> HHHHHHS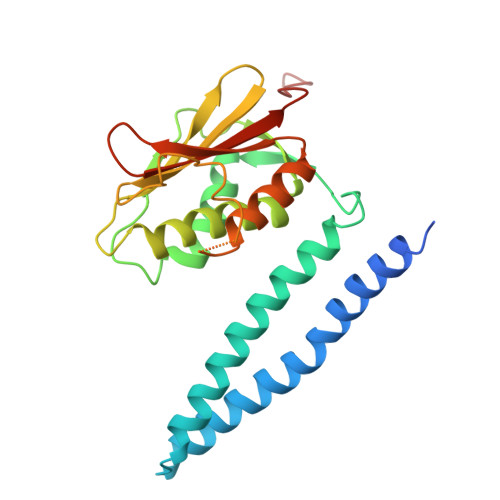SGLVPRGSHMEQIRNALLAALSHDLRTPLTVLFGQAEILTLDLASEGSPHARQASEIRQHVLNTTRLVNNLLDMARIQSGGFNLKKEWLTLEEVVGSALQMLEPGLSSPINLSLPEPLTLIHVDGPLFERVLINLLENAVKYAGAQAEIGIDAHVEGENLQLDVWDNGPGLPPGQEQTIFDKFARGNKESAVPGVGLGLAICRAIVDVHGGTITAFNRPEGGACFRVTLPQQTAPELEEFHEDM>MHHHHHHHYSYETFLKDSLELVKQVEQICGVPEALVCVM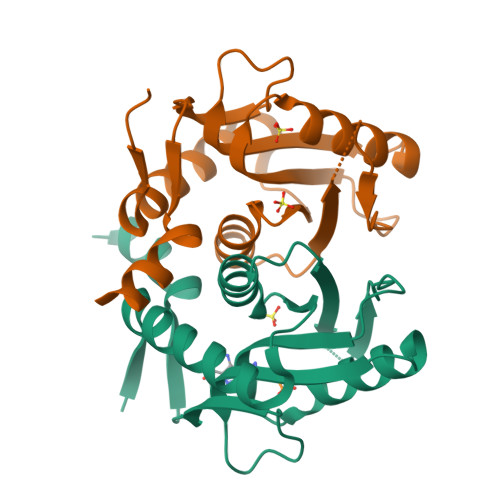RGGMTLTHFLSLHWDLREVYGINAISYDTTHRQNALKIENIPTIKDHLKTILVVDEIVDSGNSLEAVLKVLQDKHPDKKFYSASLFQKTSAKYKADAFLKDAPEWIDFFWEVDLKNLKSH[2x]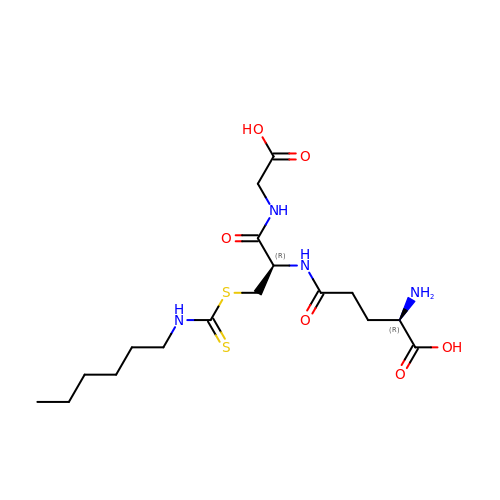(2~{R})-2-azanyl-5-[[(2~{R})-3-(hexylcarbamothioylsulfanyl)-1-(2-hydroxy-2-oxoethylamino)-1-oxidanylidene-propan-2-yl]amino]-5-oxidanylidene-pentanoic acid | C17 H30 N4 O6 S2 | XOLGYJMCQDFBBU-NEPJUHHUSA-N> DPAGLLDLRQGMFAQLVAQNVLLIDGPLSWYSDPGLAGVSLTGGLSYKEDTKELVVAKAGVYYVFFQLELRRVVAGEGSGSVSLALHL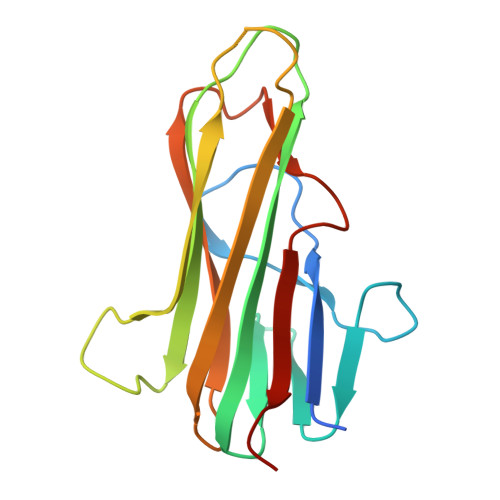QPLRSAAGAAALALTVDLPPASSEARNSAFGFQGRLLHLSAGQRLGVHLHTEARARHAWQLTQGATVLGLFRVTPEI> ANLRLSEANSGTYKTFIGRVREELGSETYRLYGIPVLKHSL;> SNRFYLLTLTSNQDESITLAIDVEDMVAVAYQPAGSHESYFFLNAPQIAFHTLFTDTHQNVLNFDNTFKSLENAAGTTRQTIVLGVDPLDFAISNLFNADPKLLPLSFLVIIQMVLEASKFRFIEQSVAYSFKNEKTFLPDLAIVSLEDNWSEISLQIQASTSLQGLFGSVVELYNSNNELIEVDSIYYPIILANVALQLYHCQVSTGD;> NECLVETRTTRISGRDALCVDVAGALTSDGSRLILYPCGQQVNQKWT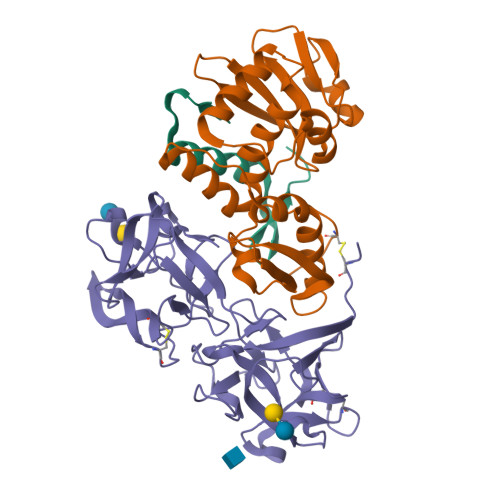FHSDGTVRSLGKCLATNNSKFGNLVVIYDCSKLAAEDISWDVSVGGTIMNPNYEDLALTSNKATRSTNLTMEVNTYSASQGWRVGNYVQPIIGSIVGLDDMCLEATDGNTNMWLEECVPNQREQSWALYSDGTIRVDDNRELCVTASSSTYDNWKVITILNCDGSNNQRWVFLADGSISTPGNQRLAMDVARSDVDLKKIILHRPHGDLNQQWVLFY> ACACGTGGACGCTGCTGCACGAG;> GTCTCGTGCAGCG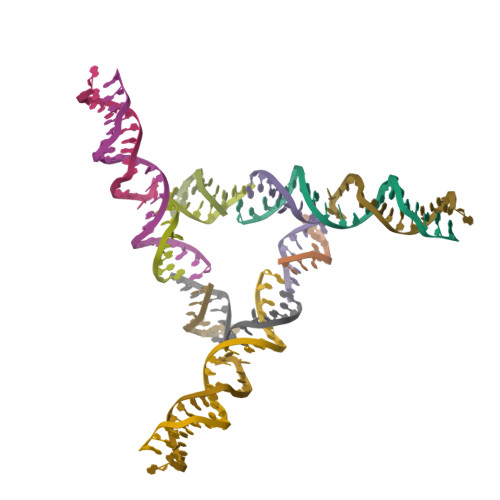TCGT;> ACTGACTC;> TGAGTCACCACGTG9-(6-DEOXY-ALPHA-L-TALOFURANOSYL)-6-METHYLPURINE | C12 H16 N4 O4 | 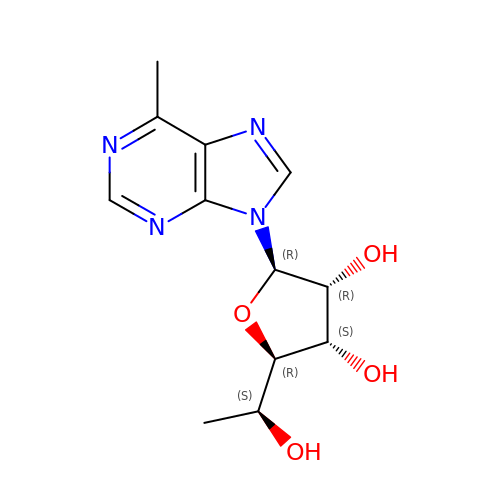XJZDIUOABWMPLZ-DSBXBFMBSA-N> MLESKLINHIATQFLDGEKDGLDSQTP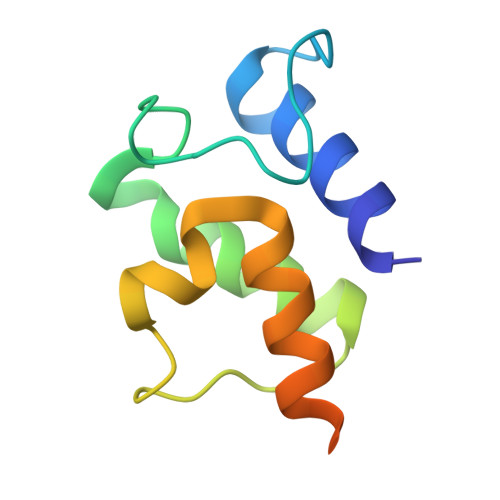LFELNIVDSAAIFDLVDFLRQESKVSIGMQEIHPANFATVQSMVALVQRLKAHPEQGGAAWEHHHHHH>[3x]GAMDMSWTDERVSTLKK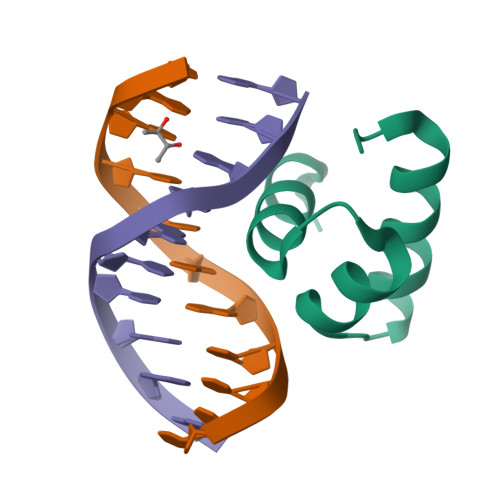LWLDGLSASQIAKQLGGVTRNAVIGKVHRLGL> SR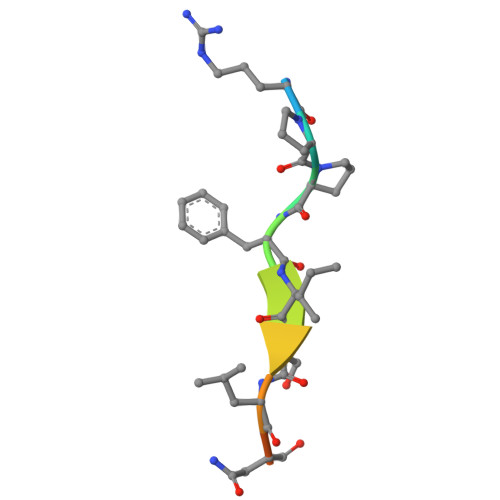PPFISLNERR> HCEGCFTSDVSSYL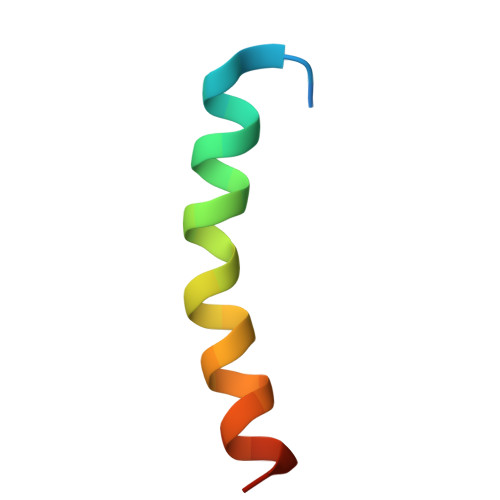EGQAAKEFIAWLVKGRG> MLERRPMAQVFDRRANTLARVSIFAGIPLVLAILGGVWWLFGWSDWHRDVGVEIPQPGGGFNHQLHVALGMDCRYCHTAVEVSAHANIPPTETCMGCHSQIISRSEKVAFVWQSWETGTSIQWNKVHDLPKFVYFNHSIHVAKGVGCSTCHGRIDQMRVVYKTQPLFMSWCLDCHRNPEKYVRPREEVFNMAWTPPPNQLEVGRRLVQEYEIRSSWELTNCAICHR;> CQFALKQPQEKIVPYVRQPEEIIHGRPLFFATAVTFAGFGVGLLVESHEGRPTKIEGNPDHPASLGSTDLITQAMILTMYDPDRSQAPTNAGQETTWDAFVAAATAAMQAQTAKQGAGLRVLSGSLTSPTLIAQKQQLLTQFPQAKWYEYEPVGRDNANAGARLAFGADVHTIYRLDTAKVIVGFDADFTAPSPTGVRMARQLADGRRIRKGTKEVNRLYLAESTPSITGLLADHRLPVRSSQIEHLVRALATLVGVPNVAAGAPLSDTEKKWVEAAAKDLQANRGACVVLVGESQPPVVHALGHAINAQLGNVGSTVVYTEPVEDDPSGGIAALSALTQEMNAGTVEVLLMIESNPVYNAPADIPFAEALAKVPLSMHVGLYRDETAQQSVWHINGAHFLEAWGDVRAFDGTTTIVQPLIAPLYNGKSAIEVLNVLLGKPQETGYQTLTAYWQTQDASGNFRVFWNTALHDGVITATQARSRQVTLQQGFADAAPPAPTQGLEIVFRPDPSLWDGAFANNAWLQETPKPYTKLTWDNVALMSVRTANALGLKNGDVVRLTYQGRSVDAPVWVQPGHADDSVTVHFGFGRTAAGRVGNNVGFNAYRLRTSATPWFGVGLEVAKVGENYKLASTQGHFLMEGRKKDLVRYGTLAEYVEDEKFLQVEKEEPISLIGEYEYNGYKWGMSIDLNVCNSCNACVVACQSENNIPVVGKDEVWLGREMHWIRIDQYYVGDEHTPNVYNMVMLCQQCEHAPCEIVCPVAATVHDAEGLNNMVYNRCVGTKYCSNNCPYKVRRFNFLQYQDVPYRSPIDASTENDSIPVLKMMRNPDVTVRARGVMEKCTFCVQRINEARIQARTENRRIADGEIMTACQQVCPTQAIVFGDLNDPQARVVDLKEQPLKYTSLDKLNTKPRVSYLAKIKNLNPDLAEEKTA;> MASQPAQKSAYGKMLEELLGPKQTYESVTRTIGDIVLTPIRKTPWGWPVGFVIAALGLLMYLFSLAVLFTVGVGVWGINIPVAWGFDIINFVWWIGIGHAGTLISAILLLFRQDWRTSINRAAEAMTIFAVACAGIYPLVHTGRPWLDYWMLPYPGTLGMWPQFRSALEWDVFAISTYATVSILFWYLGLIPDLASLRDRATNIWVKRFYGFLALGWRGGARDWNRYEVASLILAGLSTPLVLSVHSIISLDFAISQLPGWHVTVFPPYFVAGAVYCGFAMVILLLVPLRRWYKLHDL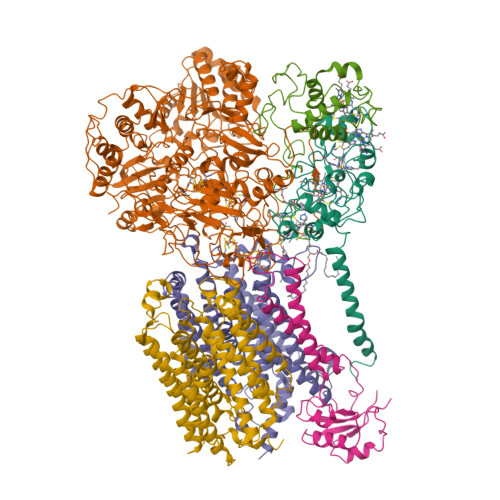ITIKHFDLMGKVMLASGLVVAYGYFAEIFYAWYSANIYEYFLITNRTMGPYAWSYWALIVLNVAIPQLLWFKRFRVSLPWLFFISICINIGMWFERWVIIVLSLHRDFLPSSWGYYTPSVWDISLYAGSFGWFFFLFFLFIRLLPAISIFEVRDLVHKTETEKALAHGSAGHH;> MLKRNARQPKALKVSTGPTLYGLMAEFDDAEALLAAAEKTRDAGYKQFEAYTPMPIHGLDEAVGYRGTRLPWVIFGAGLLGASGMFALQTWINLVEYPLNIGGRPLFSWPAFIPATFEGMVLLSAFAAVFGMIAACGLPRPYHPVFNAPNFERASVDRFFLCIEAADPKFELKQTRQFLESLGPLAVSTVDN;> XCHLEMYDQAKYKPQQASEIFADGASARPLVEHTVARGRLRIDATSTGRVDGDPNGAYVTTIPIRITPELLERGAQRYRIYCAVCHGVNGNGRGQVGLLLNPRPPSFYDQRLLDMPDGEYYDVLVNGRRTMYPYGYRVQSISDRWAIVAHIRELQKNPPPQN;> MIAQEPAALRPALGRLQQVALIVGGVAMLLAVAGAFLGAAQFFHSYIFAYFFWMALSLGGLLVLMINHLTQGVWGLMLRRLLEAAALTLPLMAILFLPIAAETLMGTHYLFPWTNPEVVANDEVVALKTPYLNVPFFLARAVIYFVLFIGMAYLLRQWSLEEDAKGFSDDLRGRFQRLSGPGIVVLVMAWTFAATDWGMSLEPEWFSSMYPVTYIASMLILTFGGGIIALAVLKSRNLLPFGIPVDRLHDLGKFLFAFVAVWAYVNFSEYLIIWSGNVPELTPWHGHRSAGGWEILGIVMIFGHFLLPFMLLLSRFAKRRLANLTAIAIYLYLIEIVWYFWKIMPAFHPDGFHIHWLDLVTLIAIGGLWLGVFAWNLQRAPLLAPNDYRVPLLRRQEASGHGHGHHGKATAEHH> MVEATAQETDRPRFSFSIAAREGKARTGTIEMKRGVIRTPAFMPVGTAATVKALKPETVRATGADIILGNTYHLMLRPGAERIAKLGGLHSFMGWDRPILTDSGGFQVMSLSSLTKQSEEGVTFKSHLDGSRHMLSPERSIEIQHLLGSDIVMAFDEVTP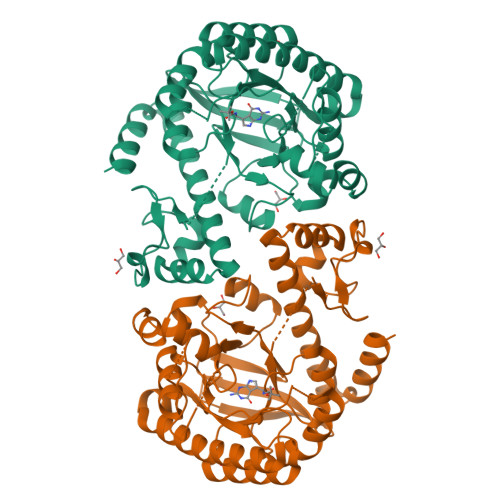YPATPSRAASSMERSMRWAKRSRDAFDSRKEQAENAALFGIQQGSVFENLRQQSADALAEIGFDGYAVGGLSGGEGQDEMFRVLDFSVPMLPDDKPHYLMGVGKPDDIVGAVERGIDMFDCVLPTRSGRNGQAFTWDGPINIRNARFSEDLKPLDSECHCAVCQKWSRAYIHHLIRAGEILGAMLMTEHNIAFYQQLMQKIRDSISEGRFSQFAQDFRARYFARNS>MEKLWLNSADSHVLEPDDLWERALPAALRDRAPRCVRDNGRETVYVDGQVVRRDPLDFADAMRPPGALDHHIRLKDLDDQGIWGEVVFPS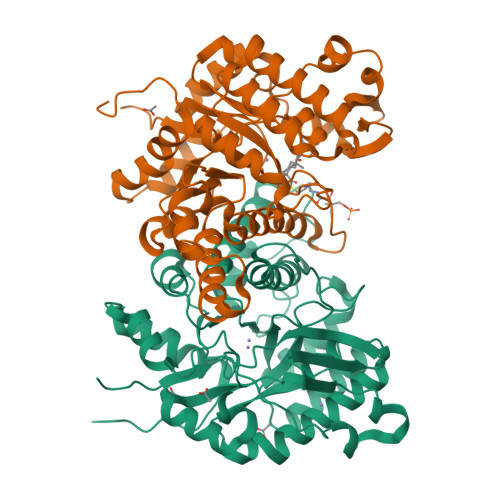RGLWTAVMTDPVLARECIKVYNDWLKSDFLSLSPRLVGAAMVSMLDTDDAVAELRRAADLGYQTVFLAATPPPGREFNMDVWEPLWAAAEEAGMTVSIHIGTGADTVVARGPGGAVINYVETLFPAQRAVAQLVASGALDRHPGLRVLIAEAGCAWVPALADRMDEAYRQHGMFVRPKLSMLPGELVRRQVYASFQHDETAIGAVTAMNYTNVLWGSDYPHLEGTFPRTQEVVTELFAGVDPEVRDLITRRNFTDLFTVPALPATV[2x]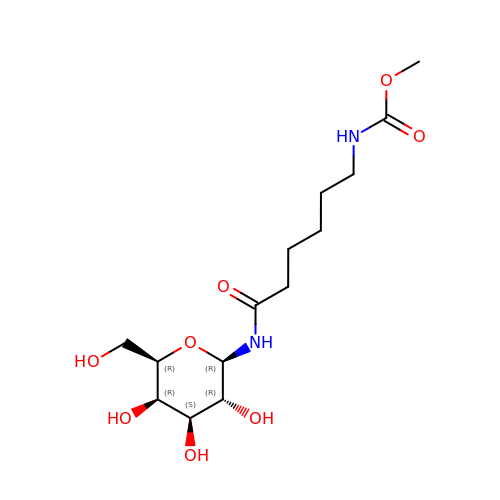[5-(3,4,5-TRIHYDROXY-6-HYDROXYMETHYL-TETRAHYDRO-PYRAN-2-YLCARBAMOYL)-PENTYL]-CARBAMIC ACID METHYL ESTER | C14 H26 N2 O8 | YTYAKGJMNHDUDF-UUWLPUTASA-N>[20x]TSVEFWQNIASGVGKWLRAIFAIAFWSSLILLTFYAIMTQVAPSKVFRLG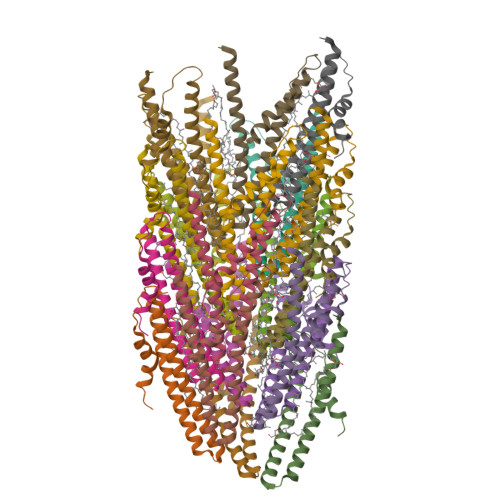ALVDLIESVKTVLLGIFVFTASVTGIIAGVAAIANAFGASFAVSPIDVVNALIFQPIVDMVK>MSEQLVTPENVTTKDGKINLLDLNRQQMREFFKDLGEKPFRADQVMKWMYHYCCDNFDEMTDINKVLRGKLKEVAEIRAPEVVEEQRSSDGTIKWAIAVGDQRVETVYIPEDDRATLCVSSQVGCALECKFCSTAQQGFNRNLRVSEIIGQVWRAAKIVGAAKVTGQRPITNVVMMGMGEPLLNLNNVVPAMEIMLDDFGFGLSKRRVTLSTSGVVPALDKLGDMIDVALAISLHAPNDEIRDEIVPINKKYNIETFLAAVRRYLEKSNANQGRVTIEYVMLDHVNDGTEHAHQLAELLKDTPCKINLIPWNPFPGAPY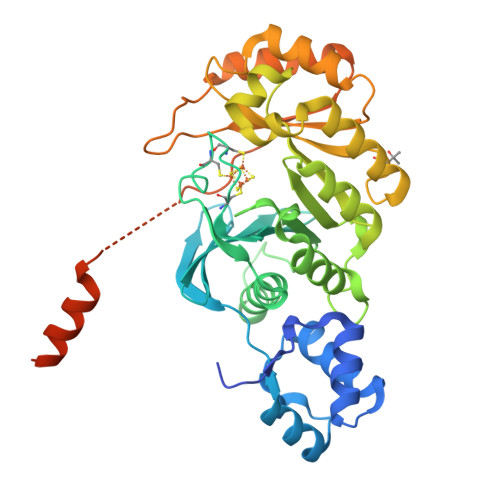GRSSNSRIDRFSKVLMSYGFTTIVRKTRGDDIDAACGQLAGDVIDRTKRTLRKRMQGEAIDIKAVGNSSSVDKLAAALEHHHHHH[2x]>MSRLPLIGVTACTKQIGLHPYHIAGDKYLRAVVNGAGGLPLIIPALGESIDQAALLDSVDGLLFTGSPSNVEPRHYSGPASEPGTLHDSDRDATTLPLVRAAIDAGIPVLGICRGFQEMNVAFGGSLHQKVHEVGTFMDHREPADQPLEVQYAPRHAMHVQPGGVLAGIGLPSEFQVNSIHGQGVDRLAP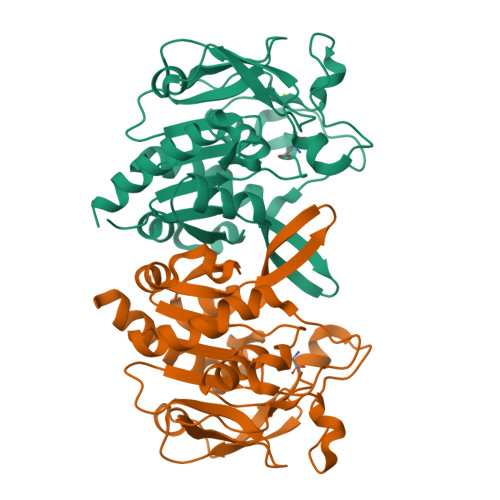GLRVEALAPDGLVEAISVEGAKAFALGVQWNPEWQVLTNPNYLAIFQAFGKACSKRAGQR[4x]> MILDADYITEDGKPVIRVFKKEKGEFKIDYDRDFEPYIYALLKDDSAIEDIKKITAERHGTTVRVTRAERVKKKFLGRPVEVWKLYFTHPQDVPAIRDKIREHPAVVDIYEYDIPFAKRYLIDRGLIPMEGDEELRMLAFDIETLYHEGEEFGEGPILMISYADEEGARVITWKNIDLPYVESVSTEKEMIKRFLKVIQEKDPDVLITYNGDNFDFAYLKKRSEMLGVKFILGRDGSEPKIQRMGDRFAVEVKGRIHFDLYPVIRRTINLPTYTLETVYEPVFGQPKEKVYAEEIARAWESGEGLERVARYSMEDAKATYELGKEFFPMEAQLSRLVGQSLWDVSRSSTGNLVEWFLLRKAYERNDVAPNKPDERELARRTESYAGGYVKEPEKGLWENIVYLDYKSLYPSIIITHNVSPDTLNREGCREYDVAPQVGHRFCKDFPGFIPSLLGDLLE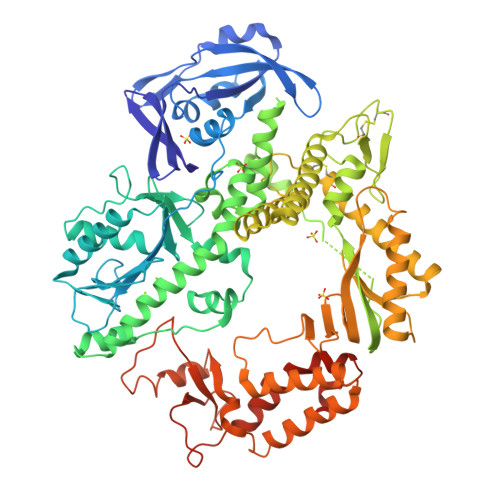ERQKVKKKMKATVDPIERKLLDYRQRAIKILANSYYGYYAYANARWYCRECAESVTAWGRQYIETTMREIEEKFGFKVLYADTDGFFATIPGADAETVKNKAKEFLNYINPRLPGLLELEYEGFYRRGFFVTKKKYAVIDEEDKITTRGLEIVRRDWSEIAKETQARVLEAILKHGDVEEAVRIVKEVTEKLSRHEVPPEKLVIYEQITRDLRSYRATGPHVAVAKRLAARGIKIRPGTVISYIVLKGPGRVGDRAIPFDEFDPAKHRYDAEYYIENQVLPAVERILRAFGYRKEDLRYQKTKQAGLGAWLKPKT>LVYSEAGPVALWLARVRWLVILILTGMVTSSILQGFESVLEAVTALAFYVPVLLGTGGNTGNQSATLIIRALATRDLDLRDWRRVFLKEMGVGLLLGLTLSFLLVGKVYWDGHPLLLPVVGVSLVLIVFFANLVGAMLPFLLRRLGVDPALVSNPLVATLSDVTGLLIYLSVARLLLE[2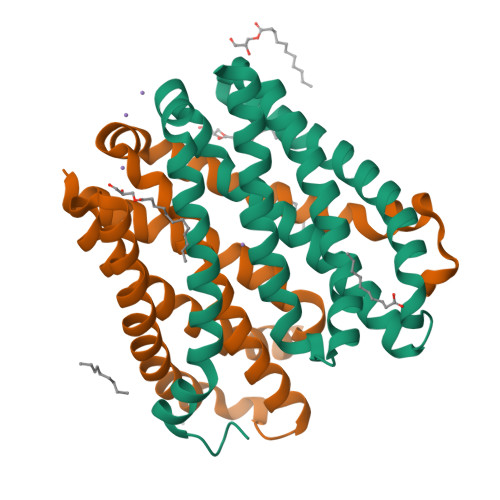x]> GHMFQCNVPLGMESGRIANEQISASSTYSDGRWTPQQSRLHGDDNGWTPNLDSNKEYLQVDLRFLTMLTAIATQGAISRETQNGYYVKSY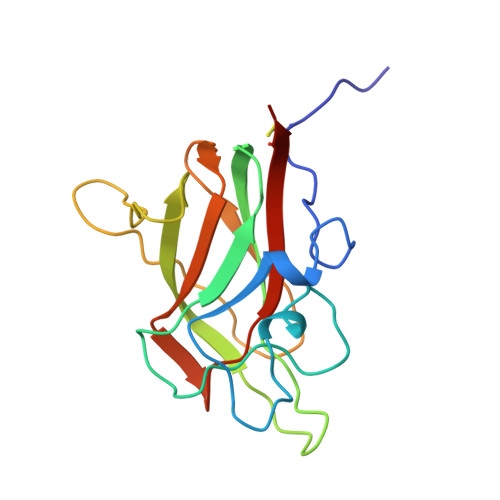KLEVSTNGEDWMVYRHGKNHKVFQANNDATEVVLNKLHAPLLTRFVRIRPQTWHSGIALRLELFGCRVTSGS Bacteriophage T5, a representative member of the T5-like family of siphophages, serves as an excellent model for studying the assembly, infection, cell wall perforation, and DNA ejection mechanisms of this phage family. In this study, we used cryo-electron microscopy (cryo-EM) to determine the structures of mature T5 (a laboratory-adapted, fiberless T5 mutant) and urea-treated empty T5 (lacking the tip complex) at near-atomic resolutions. The T5 head comprises 775 copies of MCP gp8, arranged into 11 pentons and 120 hexons, forming an icosahedral shell with a triangle number (T) of 13. The T5 tail, which comprises 40 trimeric rings of the TTP and a distal tip complex, is connected to a unique five-fold vertex of the head by the connector complex.

The distal end of the tail is occupied by the tail tip complex. We manually selected the tail tube and tail tip complexes from the micrographs by using the RELION 3.0 software and finally obtained the structures of the tail tube and tail tip complex at resolutions of 3.6 and 3.9 Å, respectively. Based on our density maps, we built atomic models of proteins p140, pb9, and pb3, as well as the C-terminus of TMP pb2 within the lumen of the tail tube tip. The tip complex contains trimeric p140, 6-fold distal tail protein pb9, and trimeric hub protein pb3. In comparison with a previously reported T5 tip complex structure, no density was observed for the three-fold side tail fiber pb1, or dodecameric collar protein p132 in our structure. One study reported the absence of p132 in the fiberless T5 (referred to as T5hd1) through Western blot detection, and this finding is consistent with that obtained from our fiberless T5 in the present study. The tail tip structures of T5, including pb9, pb3, and the C-terminus of TMP pb2, are consistent with those of the aforementioned previously reported T5 tip complex, with the exception of p140. The flexible loops of p140 at the outer surface of the tip complex exhibit slight conformational changes due to the absence of p132 and pb1 adsorption. Upon the removal of T5′s side tail fibers by mutation, the bacteriophage still forms plaques with high efficiency. Thus, as with the fiberless Lambda, T5′s side tail fibers may not be essential for the host–virus interaction to trigger the DNA release.

>[3x]MFYSLMRESKIVIEYDGRGYHFDALSNYDASTSFQEFKTLRRTIHNRTNYADSIINAQDPSSISLAINFSTTLIESNFFDWMGFTREGNSLFLPRNTPNIEPIMFNMYIINHNNSCIYFENCYVSTVDFSLDKSIPILNVGIESGKFSEVSTFRDGYTITQGEVLPYSAPAVYTNSSPLPALISASMSFQQQCSWREDRNIFDINKIYTNKRAYVNEMNASATLAFYYVKRLVGDKFLNLDPETRTPLIIKNKYVSITFPLARISKRLNFSDLYQVEYDVIPTADSDPVEINFFGERK;>[6x]MRLPDPYTNPEYPGLGFESVNLVDNDPMIRDELPNGKVKEVKISAQYWGINISYPELFPDEYAFLDSRLLEYKRTGDYLDVLLPQYEAFRVRGDTKSVTIPAGQKGSQIILNTNGTLTGQPKAGDLFKLSTHPKVYKITNFSSSGNVWNISLYPDLFITTTGSEKPVFNGILFRTKLMNGDSFGSTLNNNGTYSGISLSLRESL;>[3x]MKKILDSAKNYLNTHDKLKTACLIALELPSSSGSAATYIYLTDYFRDVTYNGILYRSGKVKSISSHKQNRQLSIGSLSFTITGTAEDEVLKLVQNGVSFLDRGITIHQAIINEEGNILPVDPDTDGPLLFFRGRITGGGIKDNVNTSGIGTSVITWNCSNQFYDFDRVNGRYTDDASHRGLEVVNGTLQPSNGAKRPEYQEDYGFFHSNKSTTILAKYQVKEERYKLQSKKKLFGLSRSYSLKKYYETVTKEVDLDFNLAAKFIPVVYGVQKIPGIPIFADTELNNPNIVYVVYAFAEGEIDGFLDFYIGDSPMICFDETDSDTRTCFGRKKIVGDTMHRLAAGTSTSQPSVHGQEYKYNDGNGDIRIWTFHGKPDQTAAQVLVDIAKKKGFYLQNQNGNGPEYWDSRYKLLDTAYAIVRFTINENRTEIPEISAEVQGKKVKVYNSDGTIKADKTSLNGIWQLMDYLTSDRYGADITLDQFPLQKVISEAKILDIIDESYQTSWQPYWRYVGWNDPLSENRQIVQLNTILDTSESVFKNVQGILESFGGAINNLSGEYRITVEKYSTNPLRINFLDTYGDLDLSDTTGRNKFNSVQASLVDPALSWKTNSITFYNSKFKEQDKGLDKKLQLSFANITNYYTARSYADRELKKSRYSRTLSFSVPYKFIGIEPNDPIAFTYERYGWKDKFFLVDEVENTRDGKINLVLQEYGEDVFINSEQVDNSGNDIPDISNNVLPPRDFKYTPTPGGVVGAIGKNGELSWLPSLTNNVVYYSIAHSGHVNPYIVQQLENNPNERMIQEIIGEPAGLAIFELRAVDINGRRSSPVTLSVDLNSAKNLSVVSNFRVVNTASGDVTEFVGPDVKLAWDKIPEEEIIPEIYYTLEIYDSQDRMLRSVRIEDVYTYDYLLTYNKADFALLNSGALGINRKLRFRIRAEGENGEQSVGWATI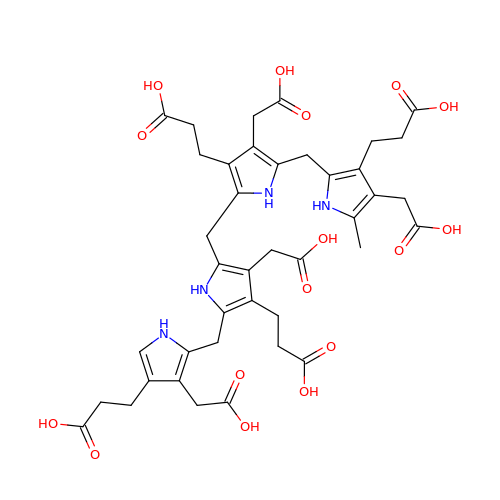3-[4-(2-hydroxy-2-oxoethyl)-5-[[4-(2-hydroxy-2-oxoethyl)-5-[[4-(2-hydroxy-2-oxoethyl)-5-[[4-(2-hydroxy-2-oxoethyl)-3-(3-hydroxy-3-oxopropyl)-5-methyl-1~{H}-pyrrol-2-yl]methyl]-3-(3-hydroxy-3-oxopropyl)-1~{H}-pyrrol-2-yl]methyl]-3-(3-hydroxy-3-oxopropyl)-1~{H}-pyrrol-2-yl]methyl]-1~{H}-pyrrol-3-yl]propanoic acid | C40 H46 N4 O16 | VHZWMEJYGVBAFI-UHFFFAOYSA-N>[4x]MGESKRTEKTRVLVVGATGYIGKRIVRACLAEGHETYVLQRPEIGLEIEKVQLFLSFKKLGARIVEGSFSDHQ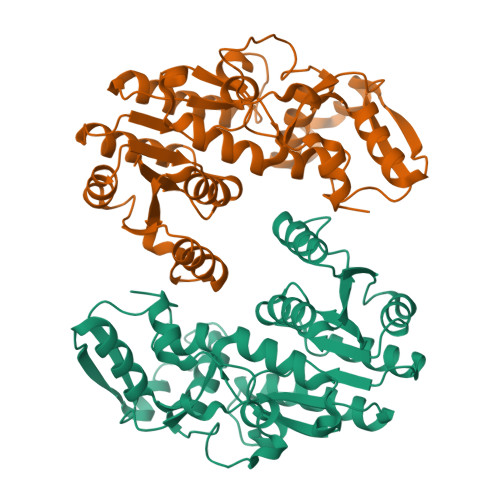SLVSAVKLVDVVVSAMSGVHFRSHNILVQLKLVEAIKEAGNVKRFLPSEFGMDPPRMGHALPPGRETFDQKMEVRQAIEAAGIPYTYVVGACFAAYFAGNLSQMVTLLPPKEKVNIYGDGNVKVVFADEDDIAKYTAKTLNDPRTLNKTVNIRPPDNVLTQLELVQIWEKLTGKELEKTNIAAQDFLANIEQMEIPHQAGIGHFYHIFYEGCLTDHEVGEDEEASSLYPDVKYKRMDDYLRMFL>SMMSPNPLQKPAIDAAPAPFADFAPPVRPQSTLRRAITAAYRRPETECLPPLVEAATQSKEIRDAAASTARKLIEALRGKHSGSGVEGLVQEYSLSSQEGVALMCLAEALLRIPDTATRDALIRDKIADGNWKSHLGGSRSLFVNAATWGLVVTGKLTSTVNDRSLAAALTRLISRCGEPVIRRGVDMAMRMMGEQFVTGETIREALKRSKELEEKGFSYSYDMLGEAATTAADAERYYRDYESAIHAIGKASAGRGIYEGPGISIKLSALHPRYSRAQAARVMGELLPRVKALALLAKNYDIGLNIDAEEADRLELSLDLLEVLCLDGDLSGWNGMGFVVQAYGKRCPFVLDFIIDLARRSGRRIMVRLVKGAYWDAEIKRAQLDGLADFPVFTRKIHTDVSYIACAAKLLAATDVVFPQFATHNAQTLAAIYHMAGKDFHVGKYEFQCLHGMGEPLYEEVVGRGKLDRPCRIYAPVGTHETLLAYLVRRLLENGANSSFVHRINDPKVSIDELIADPVEVVRAMPVVGAKHDRIALPAELFGDARTNSAGLDLSNEETLASLTEALRESAAMKWTALPQLATGPAAGETRTVLNPGDHRDVVGSVTETSEEDARRAVRLAADAAPDWAAVPPSERAACLDRAAELMQARMPTLLGLIIREAGKSALNAIAEVREAIDFLRYYAEQTRRTLGPGHGPLGPIVCISPWNFPLAIFTGQIAAALVAGNPVLAKPAEETPLIAAEGVRILREAGIPASALQLLPGDGRVGAALVAAAETAGVMFTGSTEVARLIQAQLADRLSPAGRPIPLIAETGGQNAMIVDSSALAEQVVGDVITSAFDSAGQRSSALRVLCLQEDVADRILTMLKGALHELHIGRTDRLSVDVGPVITSEAKDNIEKHIERMRGLGRKVEQIGLASETGVGTFVPPTIIELEKLSDLQREVFGPVLHVIRYRRDDLDRLVDDVNATGYGLTFGLHTRLDETIAHVTSRIKAGNLYINRNIIGAVVGVQPFGGRGLSGTGPKAGGPLYLGRLVTTAPVPPQHSSVHTDPVLLDFAKWLDGKGARAEAEAARNAGSSSALGLDLELPGPVGERNLYTLHARGRILLVPATESGLYHQLAAALATGNSVAIDAASGLQASLKNLPQTVGLRVSWSKDWAADGPFAGALVEGDAERIRAVNKAIAALPGPLLLVQAASSGEIARNPDAYCLNWLVEEVSASINTAAAGGNASLMAIG[2x]

The bifunctional enzyme proline utilization A (PutA) catalyzes the two-step oxidation of L-proline to L-glutamate using proline dehydrogenase (PRODH) and L-glutamate-γ-semialdehyde dehydrogenase (GSALDH) domains. The two active sites are 42 Å apart and connected by a buried tunnel that is hypothesized to channel the intermediates Δ1-pyrroline-5-carboxylate (P5C) and/or L-glutamate-γ-semialdehyde (GSAL). The PRODH active site is located in a (βα)8 barrel, while the GSALDH module features Rossmann NAD+-binding and catalytic domains, which are both characteristic of the ALDH superfamily. Kinetic and conventional X-ray crystallography of PutA from Sinorhizobium meliloti (SmPutA) were used to capture high resolution (1.47–1.88 Å) structures of states along the catalytic cycle, including a novel FADH−-proline covalent adduct in the PRODH site, the intermediate P5C bound noncovalently in the reduced PRODH active site, the covalent acyl-enzyme intermediate of the GSALDH reaction, and noncovalent complexes of GSAL and the final product L-glutamate in the GSALDH active site.

Catalytic cycling of the PRODH reaction was performed in crystallo by soaking crystals of the C844S variant of SmPutA in 40 mM L-proline, 1 mM Coenzyme Q1, and 1 mM NAD+. Surprisingly, the structure determined after 24 h of catalytic cycling (1.88 Å resolution) showed strong electron density evidence for a species covalently bound to the N5 of the FAD. Based on a recent quantum mechanics-molecular mechanics study of the PRODH reaction, we have modeled this species as L-proline bonded to reduced FAD. The covalent adduct links the N5 of the FAD to C5 of L-proline. The N5-C5 bond length refined to 1.66 Å, which is rather long for an N-C bond but consistent with the aforementioned quantum mechanics-molecular mechanics study. The FAD exhibits strong butterfly bending of the isoalloxazine with a bend angle of ∼20° (si face convex). Altogether, the active site in the adduct structure is partially disassembled compared to the Michaelis complex. As noted in the previous section, the covalent FADH−-proline adduct was modeled only in chain B. In chain A, electron density for the adduct was weak; however, two electron density features consistent with either proline or P5C bound noncovalently in the PRODH active site were observed. One of these features is consistent with a proline-like molecule bound noncovalently next to the si-face of the reduced FAD and was interpreted as representing a newly produced P5C molecule (occupancy of 0.73). The other site appears to be a heretofore uncharacterized secondary binding site and was interpreted as either proline entering the active site or P5C leaving (occupancy of 0.87).METYRAPONE | C14 H14 N2 O | 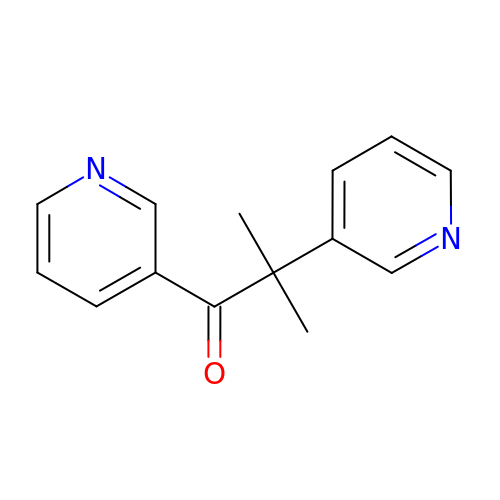FJLBFSROUSIWMA-UHFFFAOYSA-N>[2x]MIERLNSPFLRAAALFTIVAFSSLISTAALAENNPSDTAKKFKVVTTFTIIQDIAQNIAGDVAVVESITKPGAEIHDYQPTPRDIVKAQSADLILWNGMNLERWFEKFFESIKDVPSAVVTAGITPLPIREGPYSGIANPHAWMSPSNALIYIENIRKALVEHDPAHAETYNRNAQAYAEKIKALDAPLRERLSRIPAEQRWLVTSEGAFSYLAKDYGFKEVYLWPINAEQQGIPQQVRHVIDIIRENKIPVVFSESTISDKPAKQVSKETGAQYGGVLYVDSLSGEKGPVPTYISLINMTVDTIAKGFGQLEHHHHHHHHHH

The substrate-binding protein YfeA (also known as YPO2439 or y1897) is a polyspecific metal-binding protein that is crucial for nutrient acquisition and virulence in Yersinia pestis, the causative microbe of plague. Yfe is an ATP-binding cassette transporter made up of the substrate-binding protein (SBP) YfeA, the ATP-binding protein YfeB and the membrane components YfeCDE. SBPs are classified into clusters according to their three-dimensional structures and the clusters correlate with the substrate specificity. YfeA is a cluster A-I SBP that binds metal atoms such that site 1 binds Zn, Fe and Mn atoms and a secondary substrate-binding site located on the surface (site 2) binds Zn and Mn atoms.

Here, structures in which metals are inter-coordinated by multiple YfeA molecules are reported at 1.85, 2.05 and 2.25 Å resolution. The crystal structures show how a metal can bounce around site 2 and trigger distinct assemblies of protein–protein interactions. The metal recruits site 2 residues, other surface residues and His10 tag residues from multiple protomers to collaborate in metal coordination and form crystal contacts in the lattice. Three histidine residues of the His10 tag are resolved in one protomer and no histidine residues are resolved in the other protomer in the asymmetric unit. The arrangement of ligands results in square bipyramidal coordination geometry, where the His314 ligand is at the apex of the pyramid and the other four ligands form the square base. Square pyramidal coordination geometry is commonly observed in protein–manganese and protein–zinc complexes. Varied configurations of YfeA crystallographic packing show how multiple polypeptide chains can collaborate with site 2 to coordinate the metal. These configurations include a non-site-2 residue from the surrounding negative electrostatic region (YfeA site 2 inter-coordinated structure 1) or multiple site 2 motifs (structures 2 and 3).> RTEPVSTTISKSFFAPEPQIQPSFGKNVGKEGGLLFSVSLTVPENVSQVT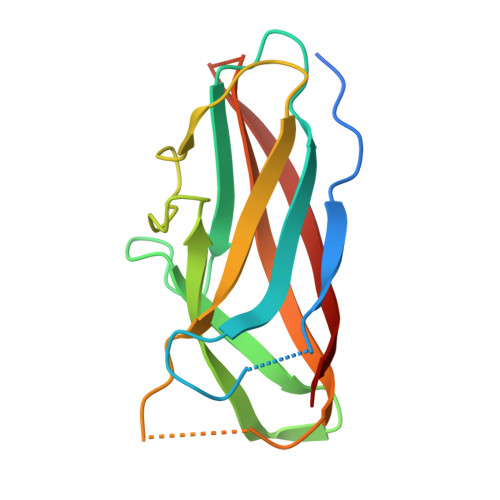VYPVYDEDYGLGRLVNTADDSQSIIYQIVDDKGRKMLKDHGAEVTPNQQITFRALNYTSGDKEIPPGIYNDQVMVGYYVNDNKQGNWQYKSLDVNVNIE Imp-L2 can bind human IGF-1, IGF-2, insulin, and DILP5 with nM affinities, it counteracts insulin signalling in Drosophila being essential for resistance to starvation, while its overexpression leads to an extension of the lifespan. Here, we report the crystal structures of the Drosophila Imp-L2 protein in its apo-form, and in holo-complexes with insect DILP5 and human IGF-1. The three-dimensional characterisation of the Imp-L2 IBP in its free and hormone-complex forms revealed its fold and hormone-binding mode that are entirely different from, and unrelated to, IGFBP-1-6. The apo-Imp-L2 consists of two, similar, immunoglobulin-(Ig)-like fold domains, each of them with two-sandwiched layers of ~6–7 anti-parallel β-strands.

The Imp-L2:DILP5 complex revealed 1:1 Imp-L2:hormone mode of binding. Imp-L2:DILP5 complex formation is correlated with the propensity of Imp-L2 to form a new type of the dimer. The crystal asymmetric unit contains here two independent, but practically identical dimers (rms of 1.0 Å), that are entirely different from the apo-Imp-L2 dimer (discussed further in detail in relation to the Imp-L2 apo→holo related quaternary transitions). The DILP5 hormone binds to Imp-L2 top id-β-sheet mainly by its B-helix that is almost perpendicular to the direction of id-β-strands. The helix runs in Ig-CT→Ig-NT direction, and is mostly engaged with the N- and C-termini part of the id-β surface. The hormone B-chain α−helix:Imp-L2 β-sheet interactions are depleted of specific, tight and directional side-chain:side-chain contacts, which are mostly of a van der Waals, hydrophobic nature over ca. ~835 Å2 buried interface. The Imp-L2 contributes βB-βE:βAC-βG-βF strands to the complex (mainly Trp32, Met58, Ile93, Leu159, Trp211, Met214, Phe233, Tyr215), while B-helix side chains are limited here to AlaB9, MetB13, ValB16, AlaB17. However, there is also more specific shape complementarity between DILP5 B-chain and the id-β-sheet as, for example, hormone MetB13 fills a hydrophobic cavity formed by Met58, Trp32, Ile93 and Leu159 of the Imp-L2. Firstly, the conformation of the N-terminus of B-chain (B1–B5) of DLP5 must change, as its extended—so-called T-like—structure, observed in its free state39 and in some insulins, would clash with the id-β-sheet surface. The positioning of the hormone on the id-β-sheet leads to a greater separation of the N- and C-termini of the Imp-L2, from ~12 Å in apo-Imp-L2, to over 20 Å distance between the Cα atoms at sites 30 and 240.

>RAVDLVDDSNDVDNSIEAEEEKPRNRAFEADWLKFTKTPPTKLQQADGATIEIVCEMMGSQVPSIQWVVGHLPRSELDDLDSNQVAEEAPSAIVRVRSSHIIDHVLSEARTYTCVGRTGSKTIYASTVVHPPRSSRLTPEKTYPGAQKPRIIYTEKTHLDLMGSNIQLPCRVHARPRAEITWLNNENKEIVQGHRHRVLANGDLLISEIKWEDMGNYKCIARNVVGKDTADTFVYPVLNEED[4x];>[4x]DFRGVVDSCCRNSCSFSTLRAYCDS;>[4x]NSLRACGPALMDMLRVACPNGFNSMFAK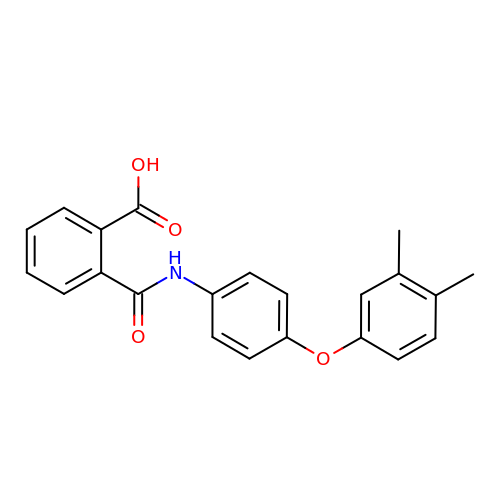2-{[4-(3,4-dimethylphenoxy)phenyl]carbamoyl}benzoic acid | C22 H19 N O4 | NZJZJKJPXZZEEC-UHFFFAOYSA-N>[2x]MRGSHHHHHHGSACELMQILLANPRGFCAGVDRAISIVENALAIYGAPIYVRHEVVHNRYVVDSLRERGAIFIEQISEVPDGAILIFSAHGVSQAVRNEAKSRDLTVFDATCPLVTKVHMEVARASRRGEESILIGHAGHPEVEGTMGQYSNPEGGMYLVESPDDVWKLTVKNEEKLSFM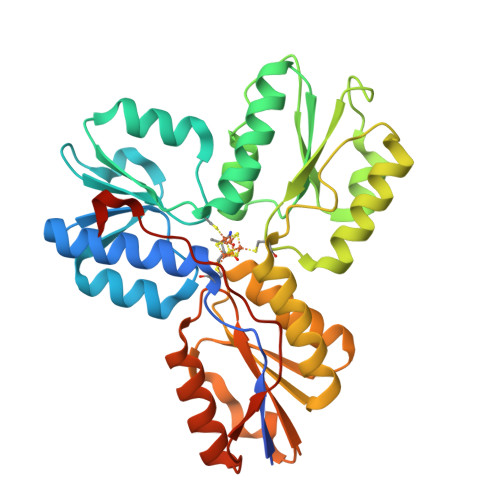TQTTLSVDDTSDVIDALRKRFPKIVGPRKDDICYATTNRQEAVRALAEQAEVVLVVGSKNSSNSNRLAELAQRMGKRAFLIDDAKDIQEEWVKEVKCVGVTAGASAPDILVQNVVARLQQLGGGEAIPLEGREENIVFEVPKELRVDIREVD> MDVSRRQFFKICAGGMAGTTVAALGFAPKQALAQARNYKLLRAKEIRNTCTYCSVGCGLLMYSLGDGAKNAREAIYHIEGDPDHPVSRGALCPKGAGLLDYVNSENRLRYPEYRAPGSDKWQRISWEEAFSRIAKLMKADRDANFIEKNEQGVTVNRWLSTGMLCASGASNETGMLTQKFARSLGMLAVDNQARVUHGPTVASLAPTFGRGAMTNHWVDIKNANVVMVMGGNAAEAHPVGFRWAMEAKNNNDATLIVVDPRFTRTASVADIYAPIRSGTDITFLSGVLRYLIENNKINAEYVKHYTNASLLVRDDFAFEDGLFSGYDAEKRQYDKSSWNYQLDENGYAKRDETLTHPRCVWNLLKEHVSRYTPDVVENICGTPKADFLKVCEVLASTSAPDRTTTFLYALGWTQHTVGAQNIRTMAMIQLLLGNMGMAGGGVNALRGHSNIQGLTDLGLLSTSLPGYLTLPSEKQVDLQSYLEANTPKATLADQVNYWSNYPKFFVSLMKSFYGDAAQKENNWGYDWLPKWDQTYDVIKYFNMMDEGKVTGYFCQGFNPVASFPDKNKVVSCLSKLKYMVVIDPLVTETSTFWQNHGESNDVDPASIQTEVFRLPSTCFAEEDGSIANSGRWLQWHWKGQDAPGEARNDGEILAGIYHHLRELYQSEGGKGVEPLMKMSWNYKQPHEPQSDEVAKENNGYALEDLYDANGVLIAKKGQLLSSFAHLRDDGTTASSCWIYTGSWTEQGNQMANRDNSDPSGLGNTLGWAWAWPLNRRVLYNRASADINGKPWDPKRMLIQWNGSKWTGNDIPDFGNAAPGTPTGPFIMQPEGMGRLFAINKMAEGPFPEHYEPIETPLGTNPLHPNVVSNPVVRLYEQDALRMGKKEQFPYVGTTYRLTEHFHTWTKHALLNAIAQPEQFVEISETLAAAKGINNGDRVTVSSKRGFIRAVAVVTRRLKPLNVNGQQVETVGIPIHWGFEGVARKGYIANTLTPNVGDANSQTPEYKAFLVNIEKA;> MAMETQDIIKRSATNSITPPSQVRDYKAEVAKLIDVSTCIGCKACQVACSEWNDIRDEVGHCVGVYDNPADLSAKSWTVMRFSETEQNGKLEWLIRKDGCMHCEDPGCLKACPSAGAIIQYANGIVDFQSENCIGCGYCIAGCPFNIPRLNKEDNRVYKCTLCVDRVSVGQEPACVKTCPTGAIHFGTKKEMLELAEQRVAKLKARGYEHAGVYNPEGVGGTHVMYVLHHADQPELYHGLPKDPKIDTSVSLWKGALKPLAAAGFIATFAGLIFHYIGIGPNKEVDDDEEDHHE;> MSKSKMIVRTKFIDRACHWTVVICFFLVALSGISFFFPTLQWLTQTFGTPQMGRILHPFFGIAIFVALMFMFVRFVHHNIPDKKDIPWLLNIVEVL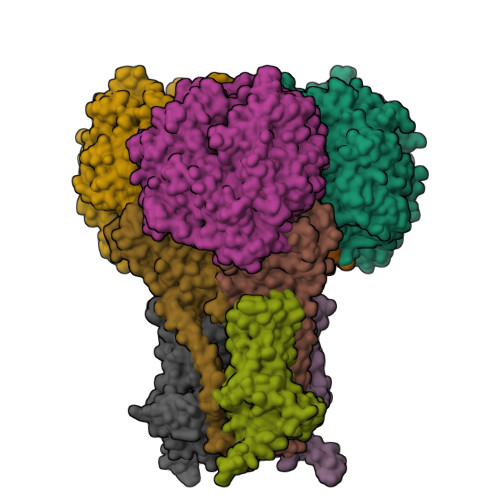KGNEHKVADVGKYNAGQKMMFWSIMSMIFVLLVTGVIIWRPYFAQYFPMQVVRYSLLIHAAAGIILIHAILIHMYMAFWVKGSIKGMIEGKVSRRWAKKHHPRWYREIEKAEAKKESEEGI> MKTIFSGIQPSGVITIGNYIGALRQFVELQHEYNCYFCIVDQHAITVWQDPH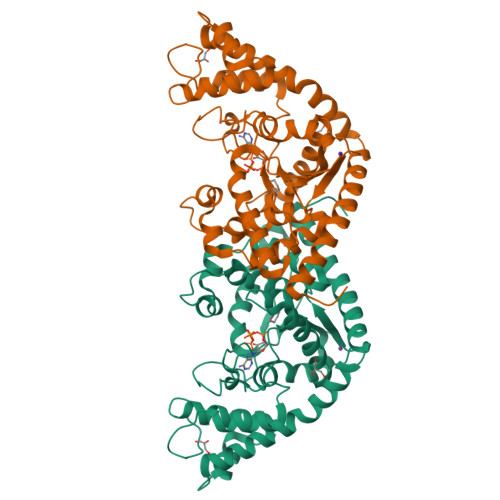ELRQNIRRLAALYLAVGIDPTQATLFIQSEVPAHAQAAWMLQCIVYIGELERMTQFKEKSAGKEAVSAGLLTYPPLMAADILLYNTDIVPVGEDQKQHIELTRDLAERFNKRYGELFTIPEARIPKVGARIMSLVDPTKKMSKSDPNPKAYITLLDDAKTIEKKIKSAVTDSEGTIRYDKEAKPGISNLLNIYSTLSGQSIEELERQYEGKGYGVFKADLAQVVIETLRPIQERYHHWMESEELDRVLDEGAEKANRVASEMVRKMEQAMGLGRRR>MKAYLVGLYTLTPTHPGSGTELGVVDQPIQRERHTGFPVIWGQSLKGVLRSYLKLVEKVDEEKINKIFGPPTEKAHEQAGLISVGDAKILFFPVRSLKGVYAYVTSPLVLNRFKRDLELAGVKNFQTEIPELTDTAIASEEITVDNKVILEEFAILIQKDDKGILESVVKAIEQAFGNEMAEKIKGRIAIIPDDVFRDLVELSTEIVARIRINAETGTVETGGLWYEEYIPSDTLFYSLILVTPRAKDNDMALIKEVLGKINGKYLQIGGNETVGKGFVKVTLKEVTNNGGTHAKHH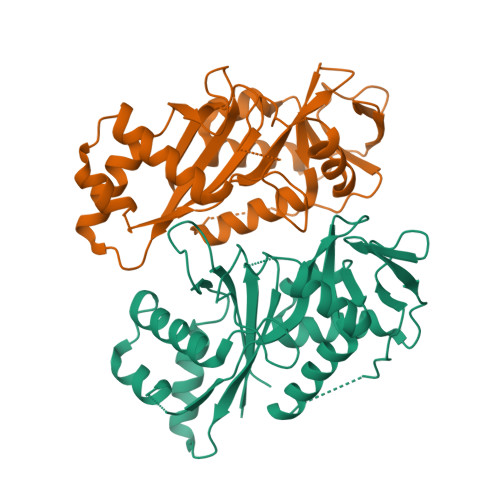HHHH[2x]> MTQAKAKHADVPVNLYRPNAPFIGKVISNEPLVKEGGIGIVQHIKFDLTGGNLKYIEGQSIGIIPPGVDKNGEPEKLRLYSIASTRHGDDVDDKTISLCVRQLEYKHPESGETVYGVCSTYLTHIEPGSEVKITGPVGKEMLLPDDPEANVIMLATGTGIAPMRTYLWRMFKDAERAANPEYQFKGFSWLVF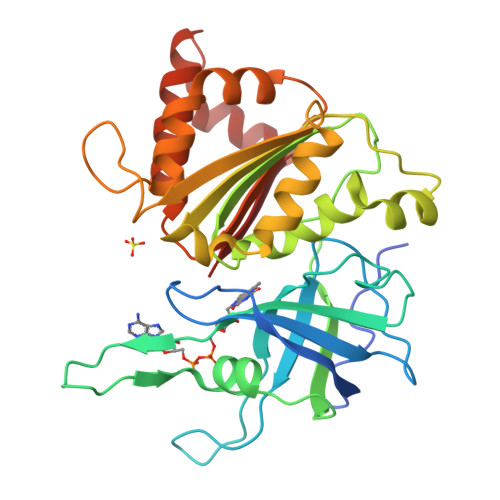GVPTTPNILYKEELEEIQQKYPDNFRLTYAISREQKNPQGGRMYIQDRVAEHADQLWQLIKNQKTHTYICGLRGMEEGIDAALSAAAAKEGVTWSDYQKDLKKAGRWHVETY>SGRFDQYPTKKGDFAIDGYLLDYSSPKQGCWVDGITVYGDIYIGKQNWGTYTRPVFAYLQYVETISIPQNVTTTLSYQLTKGHTRSFETSVNAKYSVGANIDIVNVGSEISTGFTRSESWSTTQSFTDTTEMKGPGTFVIYQVVLVYAHNATSAGRQNANAFAYSKTQAVGSRVDLYYLSAITQRKRVIVPSSNAVTP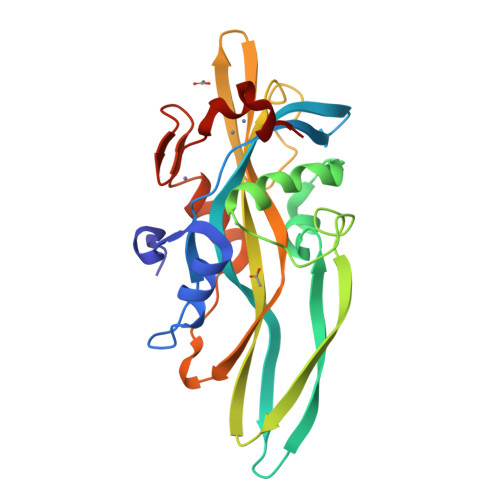LDWDTVQRNVLMENYNPGSNSGHFSFDWSAYNDPHRRY[4x]>GAMGSRKSKAELQSEERKRID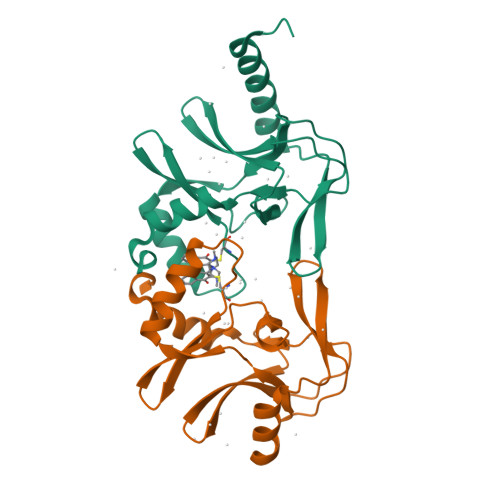ELIESGKEEGMKIDLIDGKGRGVIATKQFSRGDFVVEYHGDLIEITDAKKREALYAQDPSTGCYMYYFQYLSKTYCVDATRETNRLGRLINHSKSGNCQTKLHDIDGVPHLILIASRDIAAGEELLYDYGDRSKASIEAHPWLKH[2x]Molybdenum insertases (Mo-insertases) catalyze the final step of molybdenum cofactor (Moco) biosynthesis, an evolutionary old and highly conserved multi-step pathway. In the following synthesis steps, MPT is adenylated yielding MPT-AMP that is subsequently used as substrate for enzyme catalyzed molybdate insertion. Molybdate insertion and MPT-AMP hydrolysis are catalyzed by the Mo-insertase E-domain. The molybdate insertion reaction involves both functional domains of Mo-insertases, namely E- and G-domain whose role for the Mo-insertion reaction has been studied in detail using the plant (Arabidopsis thaliana) Mo-insertase Cnx1 as model enzyme.

We found that the conservative substitution of Cnx1E residue Asp274 by Glu (D274E) leads to an arrest of MPT-AMP hydrolysis and hence to the accumulation of MPT-AMP. We further showed that the MPT-AMP accumulation goes in hand with the accumulation of molybdate. To shed light on the molecular function of Cnx1E residue Asp274 with respect to magnesium ion coordination, we proceeded to solve the structure of the Cnx1E D274E variant. The overall structure of Cnx1E variant D274E resembles the Cnx1E wild-type structure published recently. As a notable difference, no interpretable electron density is visible in the variant structure for the region comprising amino acids 269 through 274. However, the active site magnesium ion was found to be in place. The disordered region 269 to 274 was confirmed to be highly dynamic in D274E through ensemble refinement. In the wild-type structure, residue Asp274 interacts with the octahedral water shell of the catalytically relevant magnesium ion and is therefore involved in its coordination. Replacement of Asp274 with glutamate seems to prevent this interaction and to give way to reorientation and disorder of that region. In Cnx1E wild-type, this active site loop partially covers the putative MPT-AMP binding site.

> MIPTEEALRIVFGVSKRLPPVIVSLYEALGKVLAEDIRAPDPLPPYPASVKDGYAVVASDGPGEYPVITESRAGNDGLGVTVTPGTVAYVTTGGPIPDGADAVVQVEDTKVIGDVSTESKRVKILIQTKKGTDIRRVGCDIEKDATVLTTGERIGASEIGLLATAGVTMVKVYPMPIVAILSTGDELVEPTAGTLGRGQIRDSNRAMLVAAVMQQQCKVVDLGIVRDDRKELEKVLDEAVSSGVDIILTSGGVSMGDRDFVKPLLEEKGKVYFSKVLMKPGKPLTFAEIRAKPTESMLGKTVLAFGLPGNPVSCLVCFNIFVVPTIRQLAGWTSPHPLRVRLRLQEPIKSDPIRPEFHRAIIKWKDNDGSGTPGFVAESTGHQMSSRLLSMRSANALLELPATGNVLSAGSSVSAIIVSDISAFSID> MSLSLYYKKIREQLGHELIFMPSVAAVIKNEQGELLFQYPGGEYWSLPAGAIEPGETPEEAVIREVWEETGLKVQVKKQKGVFGGKEFRYTYANGDKVEYIVVVFECEI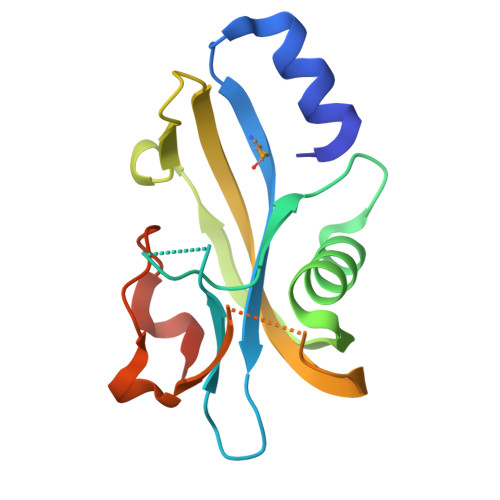TSGKLKSIDGESLKLQYFSFSEKPPLALPYPDKIFLEGHHHHHH>SMRGALQLWQFLVALLDDPTNAHFIAWTGRGMEFKLIEPEEVARLWGIQKNRPAMNYDKLSRS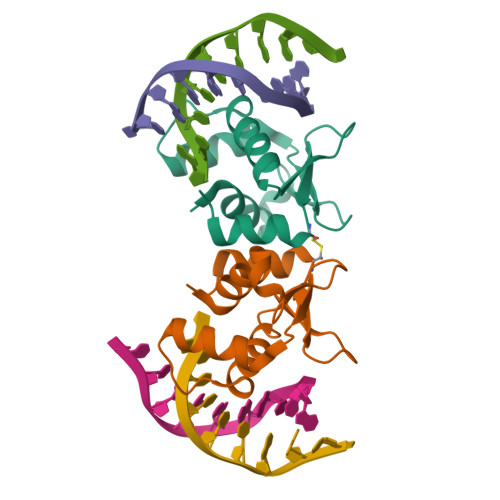LRYYYEKGIMQKVAGERYVYKFVCEPDALFSMAFPDN[8x]Mammalian cells show different susceptibilities to retrovirus infection. N-terminal β-hairpin and a core bundle of six α-helices. at positions 82, 92–94, 110, 114 and 117, can change the tropism of MLV.

tryptophan substitution at amino acid position 10 in CA. of the CA-NtD of this variant at 2.0Å resolution. RMSD of 0.6Å across equivalent Cα atoms. of the channel the aliphatic L10 side-chain forms the base. L10 in the base of the groove is shown in red. hairpin together with R112 and T107 from the α5–6 loop. residues 8 and 10 in the β-hairpin. forms part of the rhTRIM5α binding site. defined Fv1 binding pocket must be extended to include this region. observation that huTRIM5α restricted the L10W mutant virus.

> PLRLGGNGQWQYWPFSSSDLYNWKNNNPSFSEDPGKLTALIESVLTTHQPTWDDCQQLLGTLLTGEEKQRVLLEARKAVRGNDGRPTQLPNEVDAAFPLERPDWDYTTQRGRNHLVLYRQLLLAGLQNAGRSLEHHHHHH> MRRCIPARGGFTMKYKKGTGLWDEDHVNDYKTNRYLSARATMRWYQEMERHQTRNSL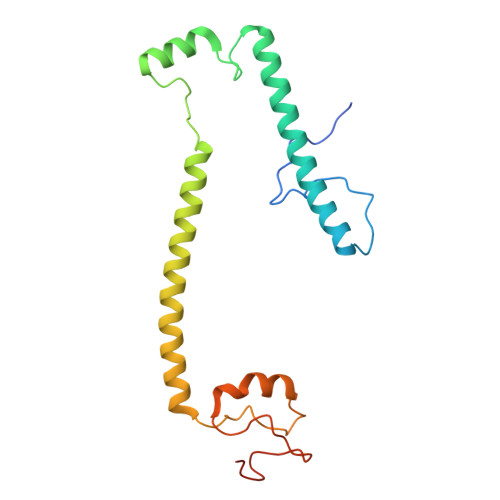NARRATQSHNNNRGLHHTGRGAFERELERRGVQVEKYPLTTTTGTMRVAELVILRRMELEKRAEEALAEQRGELQKKNPTPSEWYDESKGPLNPNFLRSMRSHYEVDIANLPDTPLIRGQREFFIGEERGNGAA> GAMGSKSQQPLQNLSHSPSYTENKPDKKKKYMINDAKTIQLVGPLISSPDNLGFQKRSHKARELPRFLINQEPQLEKRAFVQDPWDKANQEKMISLEESIDDLNELYETLKKMRNTERSIMEEKGLVDKADSAKDLYDAIVFQGTCLDMCPTFERSRRNVEYTVYSYEKNQPNDKKASRTKALKVFARPAAAAAPPLPSDVRPPHILVKTLDYIVDNLLTTLPESEGFLWDRMRSIRQDFTYQNYSGPEAVDCNERIVRIHLLILHIMVKSNVEFSLQQELEQLHKSLITLSEIYDDVRSSGGTCPNEAEFRAYALLSKIRDPQY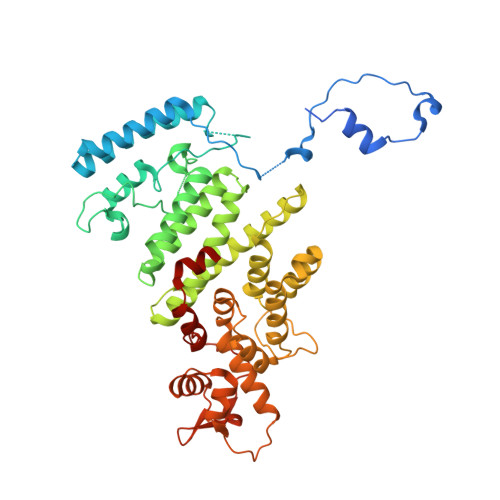DENIQRLPKHIFQDKLVQMALCFRRVISNSAYTERGFVKTENCLNFYARFFQLMQSPSLPLLMGFFLQMHLTDIRFYALRALSHTLNKKHKPIPFIYLENMLLFNNRQEIIEFCNYYSIEIINGDAADLKTLQHYSHKLSETQPLKKTYLTCLERRLQKTTYKGLINGGEDN> AKPCTVSTTNATVDLGDLYSFSLMSAGAASAWHDVALELTNCPVGTSRVTASFSGAADSTGYYKNQGTAQNIQLELQDDSGNTLNTGATKTVQVDDSSQSAHF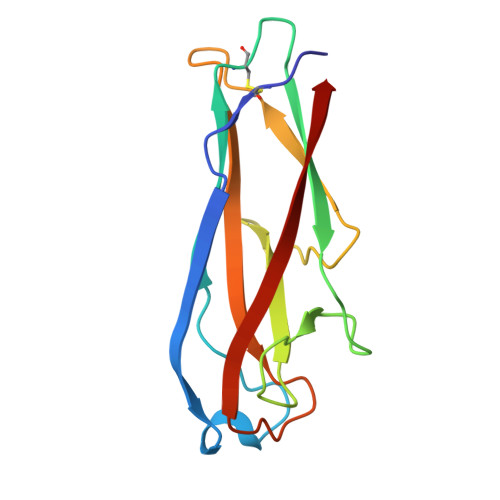PLQVRALTVNGGATQGTIQAVISITYTYS>MEIKETYDFSSIVDLWNKNIGTVYPMNLELFKQNYINDRQRK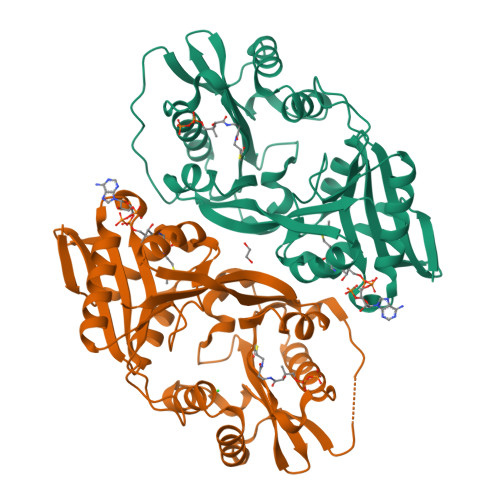KIMGAFNGEILIGFVIYKQWTYKSGSLKPNHKIGYINSIIVDINFRHQGIGTKLLDAAEEELINSGVKILRCGSDTYHFFPGIPLECLPSEEFFLVRGYKMQDYFYDLIGDVSKVDFKKPSIKDGFKVNVMKPEDRKGLFEFLEKSFSGRWLEEFIEFFQVGMKERDIVLIKYKTSVIGFSHIYDNKSSFIGPPIYWKALLGHNYGGLGPIGIDKTYRKQGLGRLLLYESLQILKKREVKKMVIDWTEKDIINFFGRFNFMPWKAYRKATKEVKDGKGGGHHHHHH[2x]> ETGVFQKAVDQSIEKKIVLRNGTEAFDSWEKPPLPVYTQFYFFNVTNPEEILRGETPRVEEVGPYTYRELRNKANIQFGDNGTTISAVSNKAYVFERDQSVGDPKIDLIRTLNIPVLTVIEWSQVHFLREIIEAMLKAYQQKLFVTHTVDELLWGYKDEILSLIHVFRPDISPYFGLFYEKNGTNDGDYVFLTGEDSYLNFTKIVEWNGKTSLDWWITDKCNMINGTDGDSFHPLITKDEVLYVFPSDFCRSVYITFSDYESVQGLPAFRYKVPAEILANTSDNAGFCIPEGN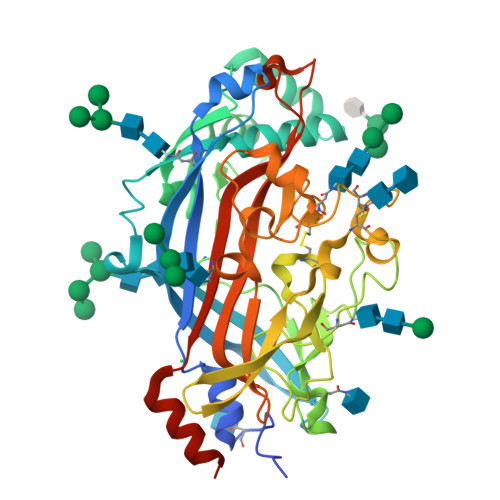CLGSGVLNVSICKNGAPIIMSFPHFYQADERFVSAIEGMHPNQEDHETFVDINPLTGIILKAAKRFQINIYVKKLDDFVETGDIRTMVFPVMYLNESVHIDKETASRLKSMINTTGKHHHHHH1-(3-pyrimidin-2-yloxyphenyl)ethanone | C12 H10 N2 O2 | 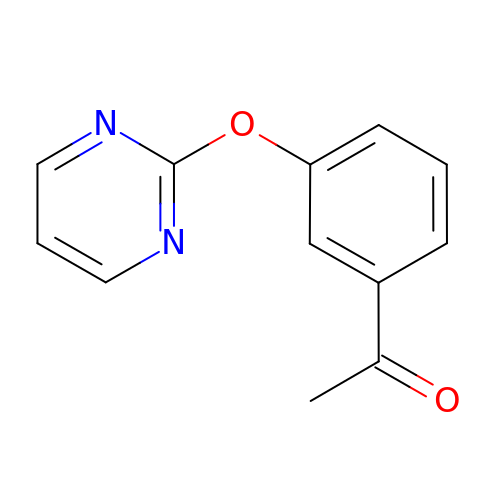OMHNTGPQUCHKHG-UHFFFAOYSA-N> MHHHHHHHHHHGENLYFQGSDNIISFDHVTFTYPDSPRPALSDLSFAIERGSWTALIGHNGSGKSTVSKLINGLLAPDDLDKSSITVDGVKLGADTVWEVREKVGIVFQNPDNQFVGATVSDDVAFGLENRAVPRPEMLKIVAQAVADVGMADYADSEPSNLSG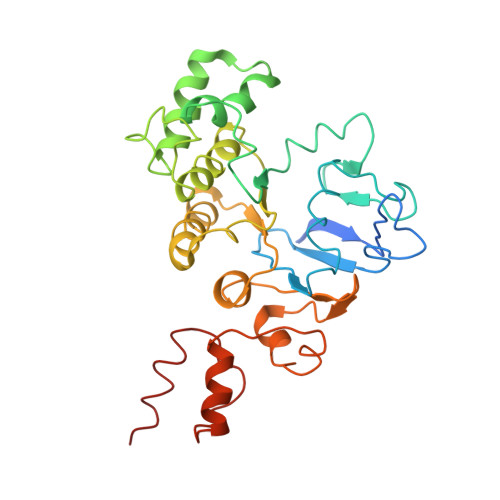GQKQRVAIAGILAVKPQVIILDESTSMLDPEGKEQILDLVRKIKEDNNLTVISITHDLEEAAGADQVLVLDDGQLLDQGKPEEIFPKVEMLKRIGLDIPFVYRLKQLLKERGIVLPDEIDDDEKLVQSLWQLNSKM>[5x]GSHMDLPTRAQMDEITSNDRPTPLANIDATDVE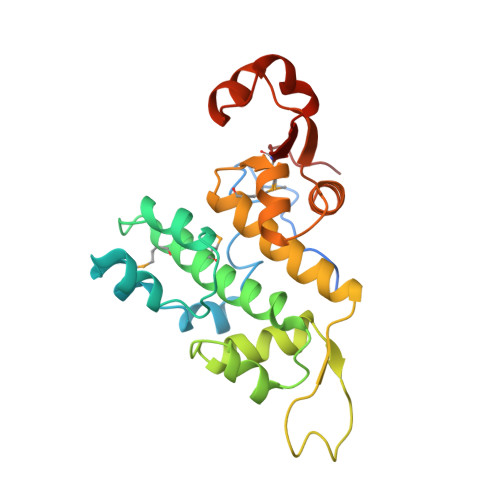QIYPIESIIPKKELQFIRVSSILKEADKEKKLELFPYQNNSKYVAKKLDSLTQPSQMTKLQMLYYLSLLLGVYENRRVNNKTKLLERLNSPPEILVDGILSRFTVIKPGQFGRSKDRSYFIDPQNEDKILCYILAIIMHLDNFIVEITPLAHELNLKPSKVVSLFRVLGAIVKGATVAQAEAFGIPKSTAASYKIATMKVPFKL>MAHHHHHHGTEKTPDDVFKLAKDEKVEYVDVRFCDLPGIMQHFTIPASAFDKSVFDDGLAFDGSSIRGFQSIHESDMLLLPDPETARIDPFRAAKTLNINFFVHDPFTLEPYSRDPRNIARKAENYLISTGIADTAYFGAEAEFYIFDSVSFDSRANGSFYEVDAISGWWNTGAATEADGSPNRGYKVRHKGGYFPVAPNDQYVDLRDKMLTNLINSGFILEKGHHEVGSGGQAEINYQFNSLLHAADDMQLYKYIIKNTAWQNGKTVTFMPKPLFGDNGSGMHCHQSLWKDGAPLMYDETGYAGLSDTARHYIGGLLHHAPSLLAFTN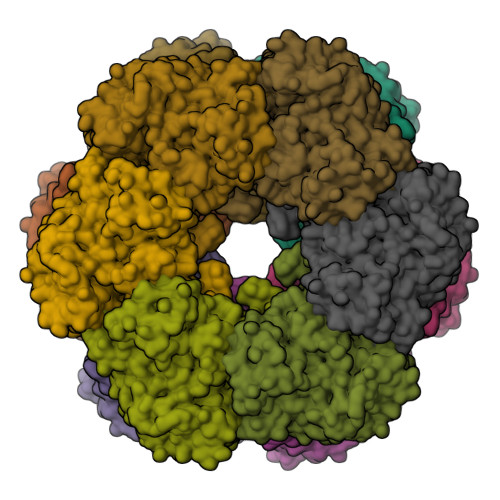PTVNSYKRLVPGYEAPINLVYSQRNRSACVRIPITGSNPKAKRLEFRSPDSSGNPYLAFSAMLMAGLDGIKNKIEPQAPVDKDLYELPPEEAASIPQTPTQLSDVIDRLEADHEYLTEGGVFTNDLIETWISFKRENEIEPVNIRPHPYEFALYYDV[6x]> VVGGV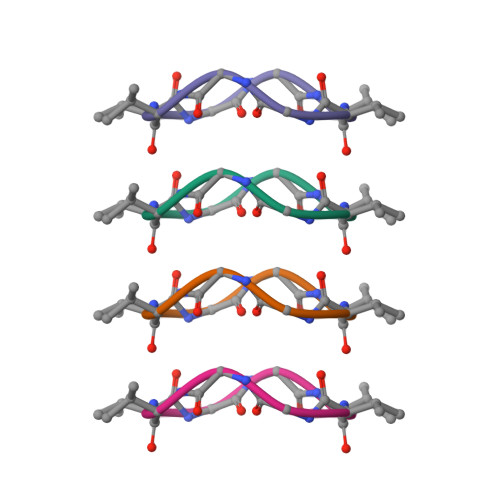VGG beta-D-arabinopyranose | C5 H10 O5 | 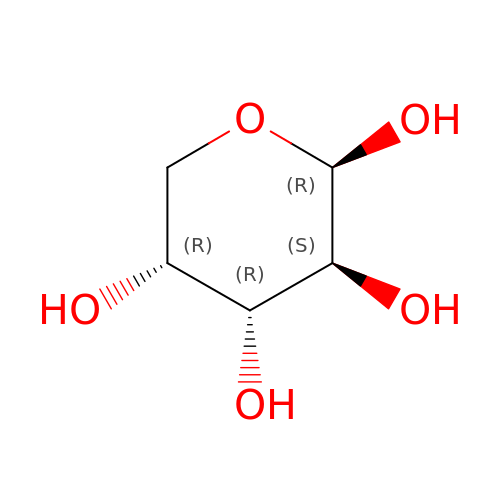SRBFZHDQGSBBOR-SQOUGZDYSA-N> MGTLYFGLSGEPSTLDTVVQPGTSGRTVKLAIHRGLVNYGIDGKISPELAESYEVSPDAKEFTFHLRQAKFHDGTTVTSADVKASLERILDPKGKASFRNELSSISKIETPDEKTVKLTLSTPSVAMIDYLALPESVIVPAAWLAKNADNPNAAPVGAGPFKFAGWTRGREITVKKFDDYYKKGKPDLDEVHYVFYSDENTRVNALKSGDVDIIDYVPAKDAADIAKGPETQLLRNTGPFMGLQFNTKFEPFSKPEVRQAIAYAVDRSAIINTAFNGLGSPIFGIAIPKGYMGYSDAKANYFSHHVEKAKALLAKAGYPN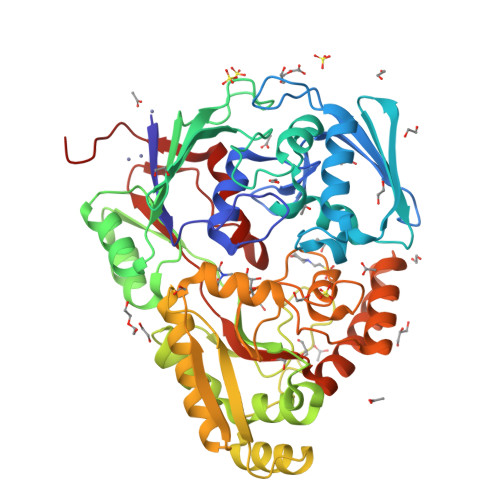GFEVRLLATSQYSFQQNTAIAIQSELAKIGIKVKLDLPDWASRMAKASTGDYDFTVMGSLGEITDADWLSNYYYGGDKLVRTNNSPYFNDQQINDLLDKGRATVDKAERVKIYDAFVDRALELSPLVYFMWREQNYAVKKGVTGFTNMPGFLTFQSGLSIENTKIEHHHHHH>LSNEDPKDALAEEWKR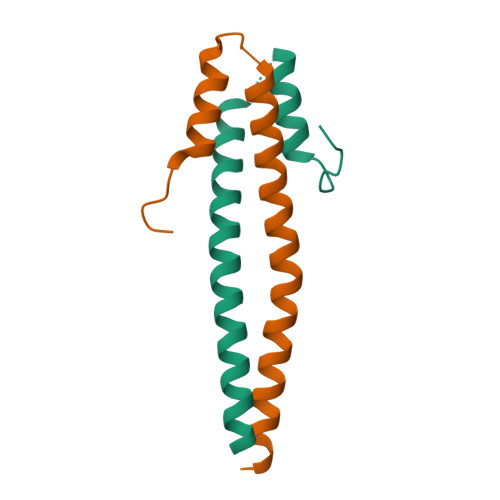RYEKEKEKVEDLEKERDFYFGKLRNIELICQENEGENDPVLQRIVDILYATDEGFVIPD[8x]> LEEKKVCQGTSNKLTQLGTFEDHFLSLQRMFNNCEVVLGNLEITYVQRNYDLSFLKTIQEVAGYVLIALNTVERIPLENLQIIRGNMYYENSYALAVLSNYDANKTGLKELPMRNLQEILHGAVRFSNNPALCNVESIQWRDIVSSDFLSNMSMDFQNHLGSCQKCDPSCPNGSCWGAGEENCQKLTKIICAQQCSGRCRGKSPSDCCHNQCAAGCTGPRESDCLVCRKFRDEATCKDTCPPLMLYNPTTYQMDVNPEGKYSFGATCVKKCPRNYVVTDHGSCVRACGADSYEMEEDGVRKCKKCEGPCRKVCNGIGIGEFKDSLSINATNIKHFKNCTSISGDLHILPVAFRGDSFTHTPPLDPQELDILKTVKEITGFLLIQAWPENRTDLHAFENLEIIRGRTKQHGQFSLAVVSLNITSLGLRSLKEISDGDVIISGNKNLCYANTINWKKLFGTSGQKTKIISNRGENSCKATGQVCHALCSPEGCWGPEPRDCVSCRNVSRGRECVDKCNLLEGEPREFVENSECIQCHPECLPQAMNITCTGRGPDNCIQCAHYIDGPHCVKTCPAGVMGENNTLVWKYADAGHVCHLCHPNCTYGCTGPGLEGCPTNGPKI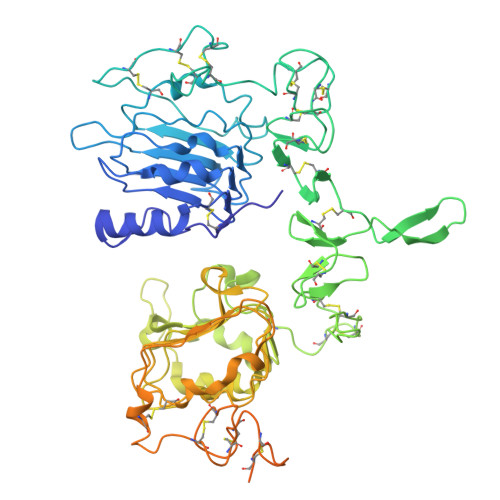PSI> MQRERLEKVMSSHTPKLDSCGAEPIHIPGAIQEHGALLVLSAREFSVVQASDNLANYIGVDLPIGAVATEANLPFISVLSAWYSGEESNFRYAWAEKKLDVSAHRSGTLVILEVEKAGVGESAEKLMGELTSLAKYLNSAPSLEDAL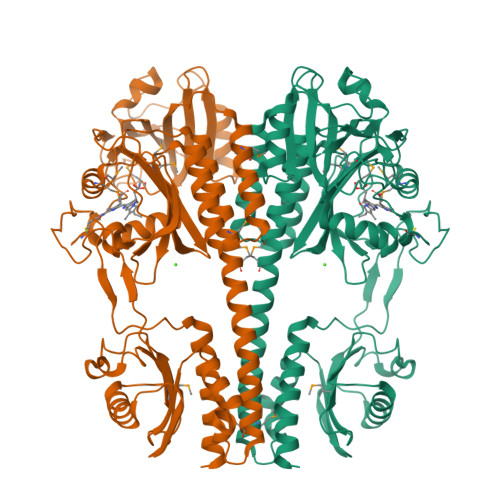FRTAQLVSSISGHDRTLIYDFGLDWSGHVVAEAGSGALPSYLGLRFPAGDIPPQARQLYTINRLRMIPDVDYKPVPIRPEVNAETGAVLDMSFSQLRSVSPVHLEYMRNMGTAASMSVSIVVNGALWGLIACHHATPHSVSLAVREACDFAAQLLSMRIAMEQSSQDASRRVELGHIQARLLKGMAAAEKWVDGLLGGEGEREDLLKQVGADGAALVLGDDYELVGNTPSREQVEELILWLGEREIADVFATDNLAGNYPTAAAYASVASGIIAMRVSELHGSWLIWFRPEVIKTVRWGGDPHKTVQESGRIHPRKSFEIWKEQLRNTSFPWSEPELAAARELRGAIIGIVLRKTEEHHHHHH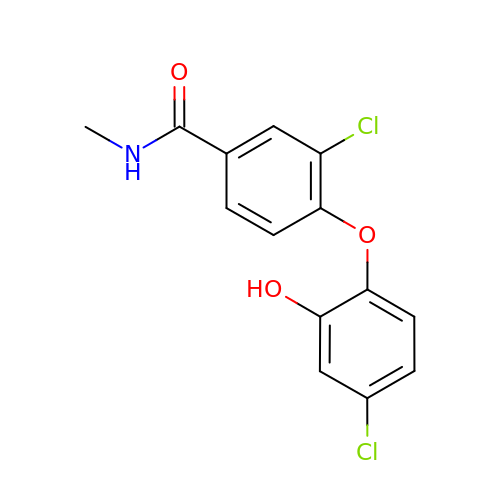3-CHLORO-4-(4-CHLORO-2-HYDROXYPHENOXY)-N-METHYLBENZAMIDE | C14 H11 Cl2 N O3 | IWVJLENCOIFPGH-UHFFFAOYSA-N N~2~-[(benzyloxy)carbonyl]-N-[(1R,2S)-1-(dihydroxyboranyl)-2-methylbutyl]-L-alaninamide | C16 H25 B N2 O5 | 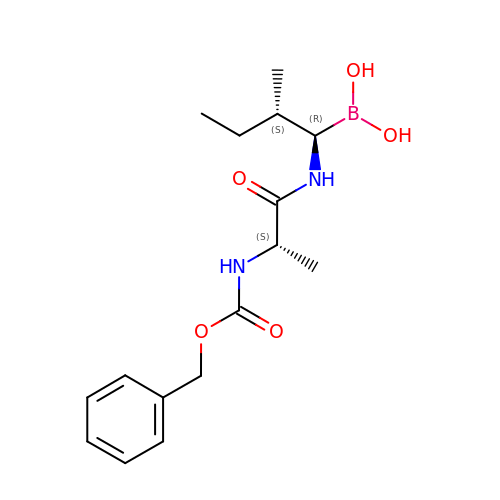WMMGWXIYADLQHX-OBJOEFQTSA-N>[2x]SACKFEEGQDVLARWSDGLFYLGTIKKINILKQSCFIIFEDSSKSWVLWKDIQTGATGSGEMVCTICQEEYSEAPNEMVICDKCGQGYHQLCHTPHIDCSVIDSDEKWLCRQCVFATTTKRGGALKKGPNAKALQVMKQTLP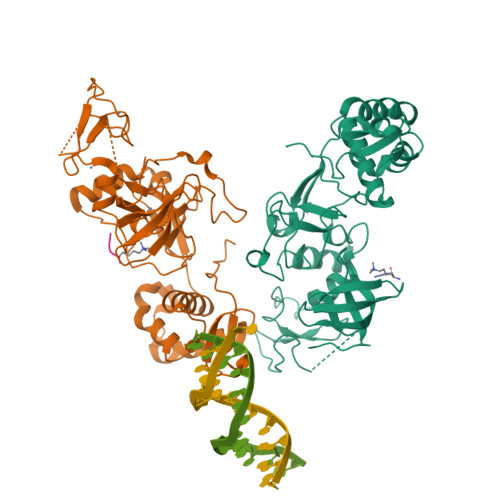YSVADLEWDAGHKTNVQQCYCYCGGPGDWYLKMLQCCKCKQWFHEACVQCLQKPMLFGDRFYTFICSVCSSGPEYLKRLPLQWVDIAHLCLYNLSVIHKKKYFDSELELMTYINENWDRLHPGELADTPKSERYEHVLEALNDYKTMFMSGKEIKKKKHLFGLRIRVPPVPPNVA;>GGVKKPHR[2x]>ASMRPVRLMKVFVTRRIPAEGRVALARAADCEVEQWDSDEPIPAKELERGVAGAHGLLCLLSDHVDKRILDAAGANLKVISTMSVGIDHLALDEIKKRGIRVGYTPDVLTDTTAELAVSLLLTTCRRLPEAIEEVKNGGWTSWKPLWLCGYGLTQSTVGIIGLGRIGQAIARRLKPFGVQRFLYTGRQPRPEEAAEFQAEFVSTPELAAQSDFIVVACSLTPATEGLCNKDFFQKMKETAVFINISRGDVVNQDDLYQALASGKIAAAGLDVTSPEPLPT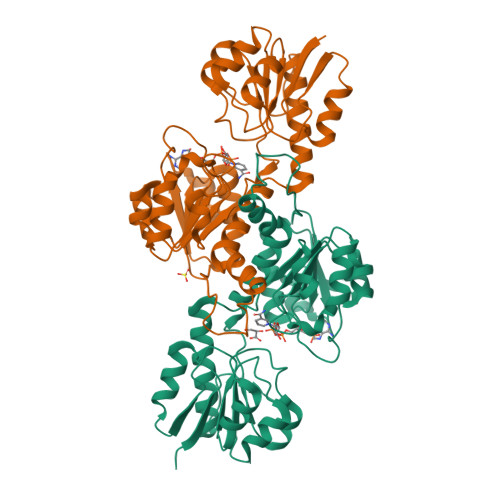NHPLLTLKNCVILPHIGSATHRTRNTMSLLAANNLLAGLRGEPMPSELKL[4x]Amylomaltase (AM, EC 2.4.1.25) is an intracellular 4-αGTase that catalyzes the intermolecular (disproportionation, coupling, hydrolysis) and intramolecular (cyclization) transglycosylation reactions to yield new linear oligosaccharides and LR-CD or cycloamylose (CA) products, respectively. In the present work, a novel AM from the mesophilic bacterium Streptococcus agalactiae (SaAM), with 18–49% sequence identity to previously reported AMs, was characterized. SaAM has the conserved catalytic and substrate recognition residues (D295, E342 and D396, SaAM numbering), which are found in all AMs. SaAM is phylogenetically grouped with AMs from the mesophilic bacteria, but has a similar size to AMs of the thermophiles.

Therefore, we determined the X-ray crystal structure of SaAM in complex with acarbose to gain an insight into its thermostability and catalytic mechanism. Eight chains of SaAM were identified in the asymmetric unit, and the results showed that all chains are similar. We found two ligands present in the active site. The first ligand is an acarbose molecule that had reacted with the catalytic nucleophile D295, cleaving off a glucose residue at the reducing end, resulting in an acarbose-derived glycosyl-enzyme intermediate at D295. The second ligand is an intact acarbose molecule close to the glycosyl-enzyme intermediate. The 4-OH group of the non-reducing end of the second acarbose molecule is around 3.9 Å away from the anomeric carbon atom of the glycosyl-enzyme intermediate. Therefore, we believe that we have captured the pre-transglycosylation step of the catalytic mechanism with the acarbose molecule resembling a non-reducing end attacking the glycosyl-enzyme intermediate. The alkene moiety in the non-reducing end may have caused the 4-OH to be in a sub-optimal position for nucleophilic attack, thus allowing isolation of the catalytic intermediate. The interactions of the enzyme with the 2-OH and 3-OH groups of the non-reducing end help position the 4-OH for nucleophilic attack and also block the 2-OH and 3-OH groups from reacting with the glycosyl-enzyme intermediate. Thus, our novel structure also explains the regioselectivity of the transglycosylation reaction.

>[8x]MAKKRASGVLMHITSLPGDLGIGTFGREAYAFVDFLVETDQKFWQILPLTTTSFGDSPYQSFSAVAGNTHLIDFDLLTLEGFISKDDYQNISFGQDPEVVDYAGLFEKRRPVLEKAVKNFLKEERATRMLSDFLQEEKWVTDFAEFMAIKEHFGNKALQEWDDKAIIRREEEALAGYRQKLSEVIKYHEVTQYFFYKQWFELKEYANDKGIQIIGDMPIYVSADSVEVWTMPELFKLDRDKQPLAIAGVPADDFSDDGQLWGNPIYNWDYHKESDFDWWIYRIQSGVKMYDYLRIDHFKGFSDYWEIRGDYQTANDGSWQPAPGPELFATIKEKLGDLPIIAENLGYIDERAERLLAGTGFPGMKIMEFGFYDTTGNSIDIPHNYTENTIAYAGTHDNEVINGWFENLTVEQKAYAENYMRRLPNEPITETVLRTLYATVSQTTITCMQDLLDKPADSRMNMPNTVGGNWQWRMRKEDLTENRKAFLKEITTIYNRGNKLEHHHHHH>MKGPNLNFRKTPSKDNGVKQVESLARPETPPPKFVEDSNLEFNVLASEKLPNYTNLDLFHRAVFPFMFLAQCVAIMPLVGIRESNPRRVRFAYKSIPMFVTLIFMIATSILFLSMFTHLLKIGITAKNFVGLVFFGCVLSAYVVFIRLAKKWPAVVRIWTRTEIPFTKPPYEIPKRNLSRRVQLAALAIIGLSLGEHALYQVSAILSYTRRIQMCANITTVPSFNNYMQTNYDYVFQLLPYSPIIAVLILLINGACTFVWNYMDLFIMMISKGLSYRFEQITTRIRKLEHEEVCESVFIQIREHYVKMCELLEFVDSAMSSLILLSCVNNLYFVCYQLLNVFNKLRWPI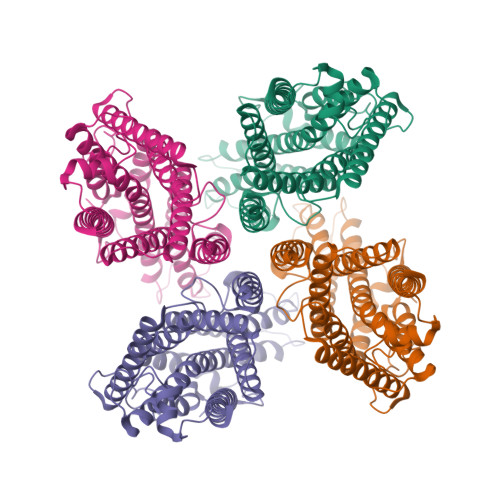NYIYFWYSLLYLIGRTAFVFLTAADINEESKRGLGVLRRVSSRSWCVEVERLIFQMTTQTVALSGKKFYFLTRRLLFGMAGTIVTYELVLLQFDEPNRRKGLQPLCALEGGSSGGWSHPQFEK[4x]>GPKITLLTLIKTAEHWARQDIRTIEDSKLRALLTLCAVMTRKFSKSQLSLLCETHLRREGLGQDQAEPVLEVYQRLHSDKGGSFEAALW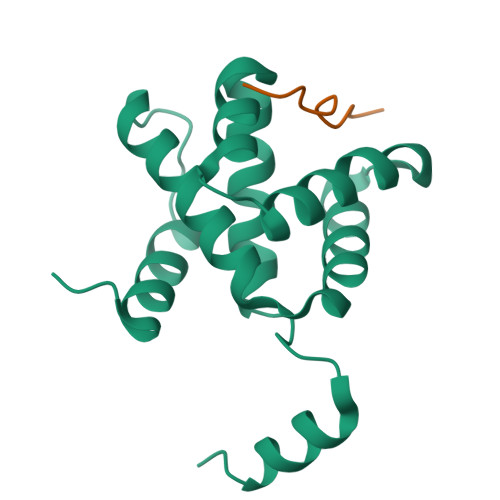QQWDRQSLIMFITAFLNIALQLPCESSAVVVSGLRTLVPQ[4x];>PTVAPPAPVYR[4x]2-butyl[1,3]oxazolo[4,5-c]quinolin-4-amine 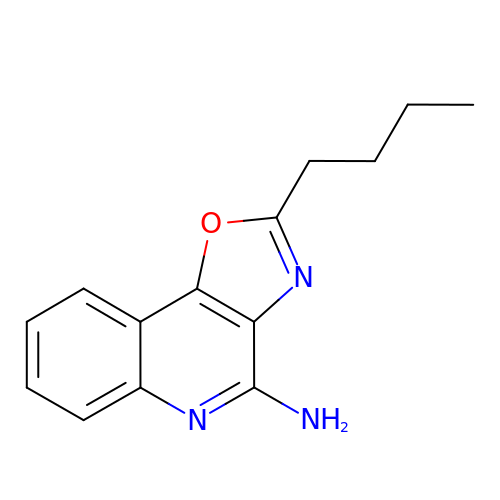| C14 H15 N3 O | XGNXMXDDPAAWFU-UHFFFAOYSA-N> SMDNQCTVQVRLELGHRAQLRKKPTTEGFTHDWMVFVRGPEQCDIQHFVEKVVFWLHDSFPKPRRVCKEPPYKVEESGYAGFIMPIEVHFKNKEEPRKVCFTYDLFLNLEGNPPVNHLRCEKLT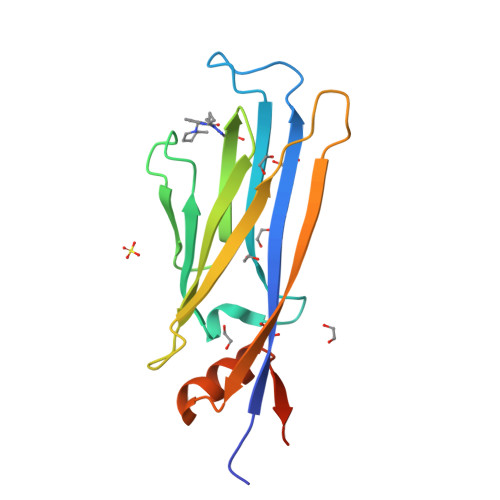FNNPTTEFRYKLLRAGGVMVMPEGAHHHHHH> PGMMDS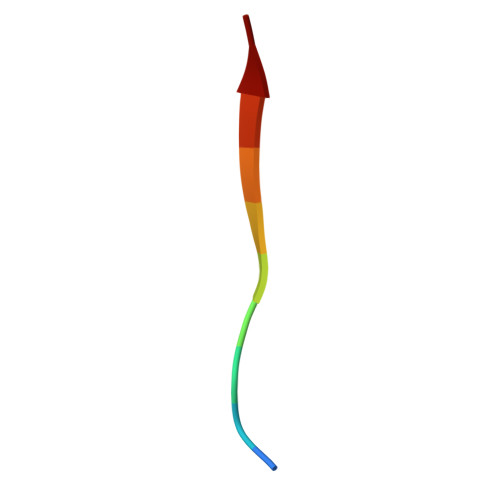QEFS> MAFVSGAGAAVRGTSGKAAARCAAVRTVRAARAIRMTTAPGSAPFSSLDEPERQVVMWESVGDEKDQVFKQLYRQVFGNAYLMESDLEELLVPESQLLMGSISVKDFIKRVAKSDAYKKRFFE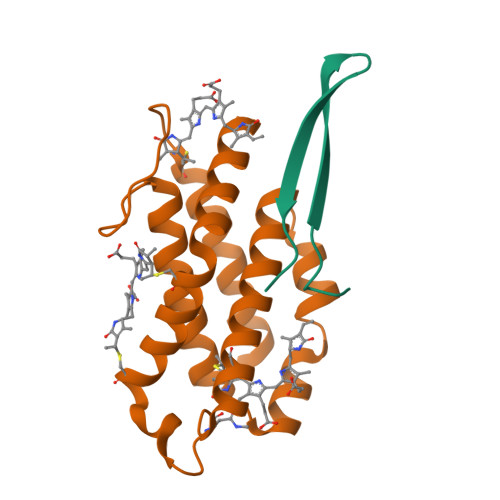PCGPYRFVELCTKHFLGRGPRDQKEVSEHVQRLANEGYDADVDSYMDSEEYMSLFGENGVPRFVFKGTYEGNDQFNRLAAMRQFADGSYTDTRSGSTAPRKAQKAELTMAEGDFVGRAKVSRGLPAETSAAKTGTPPVRALKGPVNPRAGVRVRIKVVDNLYQVYEIPPMADPKAKVNAFWAKPIPSSLTKKY;> MLDAFSRVVVNSDAKAAYVGGSDLQALKSFIADGNKRLDAVNSIVSNASCMVSDAVSGMICENPGLISPGGNCYTNRRMAACLRDGEIILRYVSYALLAGDASVLEDRCLNGLKETYIALGVPTNSSIRAVSIMKAQAVAFITNTATERKMSFAAGDCTSLASEVASYFDRVGAAIS>[2x]MKFLKNVLEEGSKLEEFNELELSPEDKELLEYLQQTKAKITVVGCGGAGNNTITRLKMEGIEGAKTVAINTDAQQLIRTKADKKILIGKKLTRGLGAGGNPKIGEEAAKESAEEIKAAIQDSDMVFITCGLGGGTGTGSAPVVAEISKKIGALTVAVVT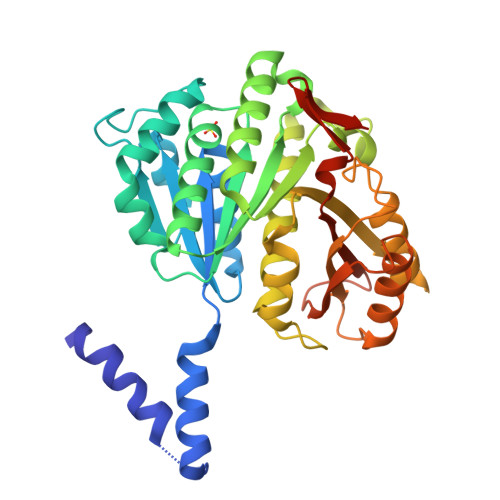LPFVMEGKVRMKNAMEGLERLKQHTDTLVVIPNEKLFEIVPNMPLKLAFKVADEVLINAVKGLVELITKDGLINVDFADVKAVMNNGGLAMIGIGESDSEKRAKEAVSMALNSPLLDVDIDGATGALIHVMGPEDLTLEEAREVVATVSSRLDPNATIIWGATIDENLENTVRVLLVITGVQSRIEFTDTGLKRKKLELTGIPKI>GPDRSFRWKYHQFRFLCHSNALPSHVKISVSRQTLFEDSFQQIMNMKPYDLRRRLYIIMRGEEGLDYGGIAREWFFLLSHEVLNPMYCLFEYAGKNNYCLQINPASSINPDHLTYFRFIGRFIAMALYHGKFIDTGFTLPFYKRMLNKRPTLKDLESIDPEFYNSIVWIKENNLEECGLELYFIQDMEILGKVTTHELKEGGESIRVTEENKEEYIMLLTDWRFTRGVEEQTKAFLDGFNEVAPLEWLRYFDEKELELMLCGMQEIDMSDWQKSTIYRHYTKNSKQIQWFWQVVKEMDNEKRIRLLQFVTGTCRLPVGGFAELI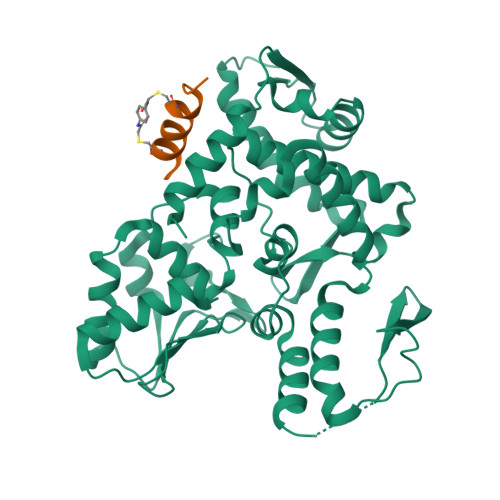GSNGPQKFCIDKVGKETWLPRSHTCFNRLDLPPYKSYEQLREKLLYAIEETE[2x];>XDPATIMCRAAADTCTFFX[2x]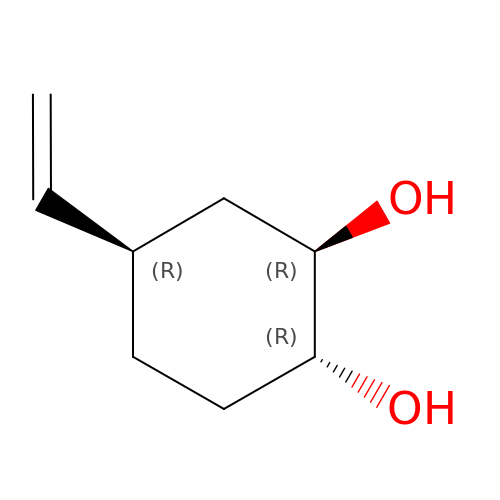(1R,2R,4R)-4-ethenylcyclohexane-1,2-diol | C8 H14 O2 | BSJHRRSHDADBTA-OECOWPMFSA-N> TLSILVAHDLQRVIGFENQLPWHLPNDLKHVKKLSTGHTLVMGRKTFESIGKPLPNRRNVVLTSDTSFNVEGVDVIHSIEDIYQLPGHVFIFGGQTLF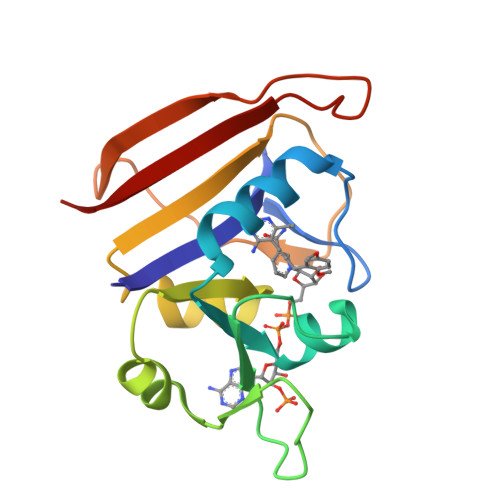EEMIDKVDDMYITVIEGKFRGDTFFPPYTFEDWEVASSVEGKLDEKNTIPHTFLHLIRK> GSMAEQATKSVLFVCLGNICRSPIAEAVFRKLVTDQNISENWRVDSAATSGYEIGNPPDYRGQSCMKRHGIPMSHVARQITKEDFATFDYIL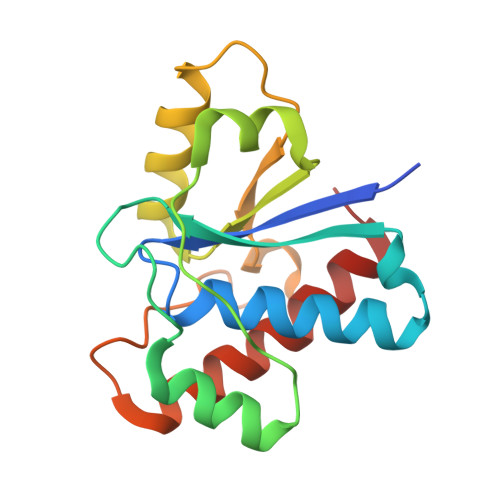CMDESNLRDLNRKSNQVKTCKAKIELLGSYDPQKQLIIEDPYYGNDSDFETVYQQCVRCCRAFLEKAH> MAGGEAGVTLGQPHLSRQDLTTLDVTKLTPLSHEVISRQATINIGTIGHVAHGKSTVVKAISGVHTVRFKNELERNITIKLGYANAKIYKLDDPSCPRPECYRSCGSSTPDEFPTDIPGTKGNFKLVRHVSFVDCPGHDILMATMLNGAAVMDAALLLIAGNESCPQPQTSEHLAAIEIMKLKHILILQNKIDLVKESQAKEQYEQILAFVQGTVAEGAPIIPISAQLKYNIEVVCEYIVKKIPVPPRDFTSEPRLIVIRSFDVNKPGCEVDDLKGGVAGGSILKGVLKVGQEIEVRPGIVSKASEGKLMCKPKFSKIVSLFAEHNDLQYAAPGGLIGVGTKIDPTLCRADRMVGQVLGAVGALPEIFTELEISYFLLRRLLGVRTEGDKKAAKVQKLSKNEVLMV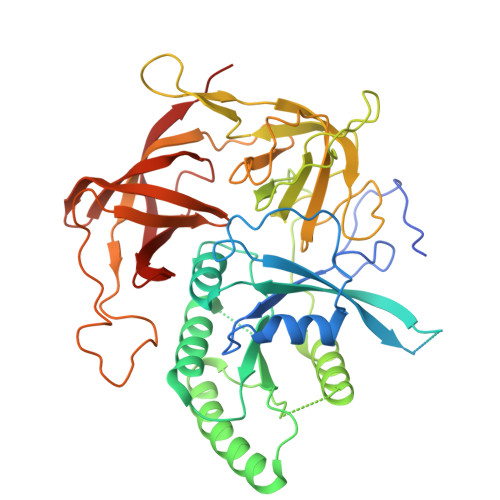NIGSLSTGGRVSAVKADLGKIVLTNPVCTEVGEKIALSRRVEKHWRLIGWGQIRRGVTIKPTVDDD> VEFGSMPPKRRLVDDADAMEDQDLYEPPASLPKLPGKFLQYTVGGSDPHPGIGHEKDIRQNAVALLDQSRRDMFHTVTPSLVFLCLLIPGLHAAFVHGGVPRESYLSTPVTRGEQTVVKTAKFYGEKTTQRDLTELEISSIFSHCCSLLIGVVIGSSSKIKAGAEQIKKRFKTMMAALNRPSHGETATLLQMFNPHEAIDWINGQPWVGSFVLSLLTTDFESPGKEFMDQIKLVASYAQMTTYTTIKEY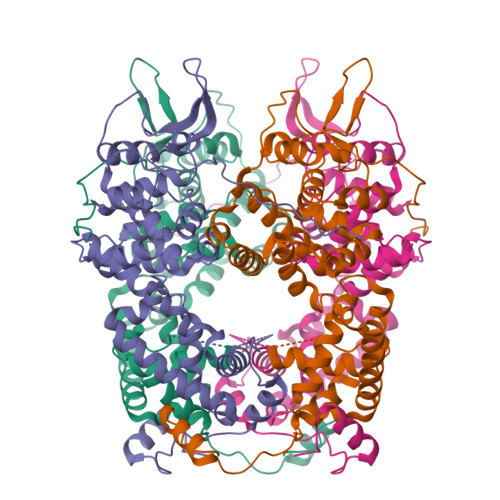LAECMDATLTIPVVAYEIRDFLEVSAKLKEDHADLFPFLGAIRHPDAIKLAPRSFPNLASAAFYWSKKENPTMAGYRASTIQPGASVKETQLARYRRREISRGEDGAELSGEISAIMKMIGVTGLN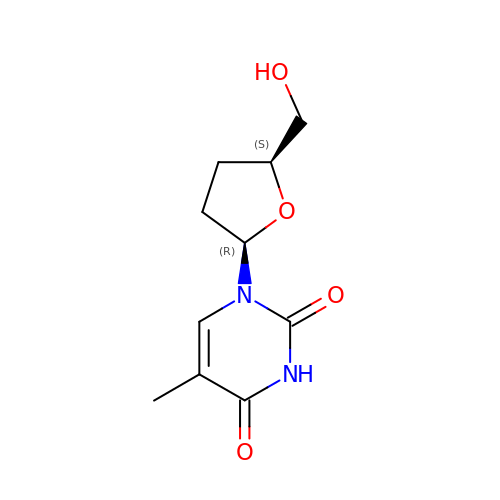1-[(2R,5S)-5-(hydroxymethyl)tetrahydrofuran-2-yl]-5-methylpyrimidine-2,4(1H,3H)-dione | C10 H14 N2 O4 | XKKCQTLDIPIRQD-JGVFFNPUSA-N>MPIITDVYAREVLDSRGNPTVEVEVLTESGAFGRALVPSGASTGEHEAVELRDGDKSRYLGKGVTKAVENVNEIIAPEIIEGEFSVLDQVSIDKMMIALDGTPNKGKLGANAILGVSIAVARAAADLLGQPLYKYLGGFNGKQLPVPMMNIVNGGSHSDAPIAFQEFMILPVGATTFKESLRWGTEIFHNLKSILSKRGLETAVGDEGGFAPKFEGTEDAVETIIQAIEAAGYKPGEEVFLGFDCASSEFYENGVYDYSKFEGEHGAKRTAAEQVDYLEQLVDKYPIITIEDGMDENDWDGWKQLTERIGDRVQLVGDDLFVTNTEILAKGIENGIGNSILIKVNQIGTLTETFDAIEMAQKAGYTAVVSHRSGETEDTTIADIAVATNAGQIK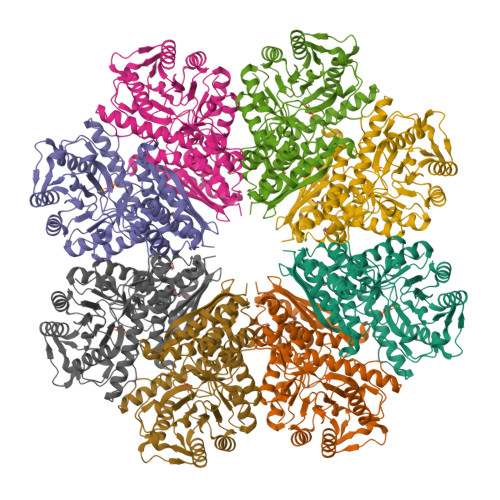TGSLSRTDRIAKYNQLLRIEDELFETAKYDGIKSFYNLDKLEHHHHHH[2x]> DRPAVVHSVRALMLAERQGGGGSGGGGSGGGGSFFYGKIGECHYLNGTERVRFLDRQIYNRQQFAHFDSDVGKFVADTPLGEPQAEYWNSNAELLENLMNEVDRVCRHNYGILESFTVQRSVEPKVRVSALQSGSLPETD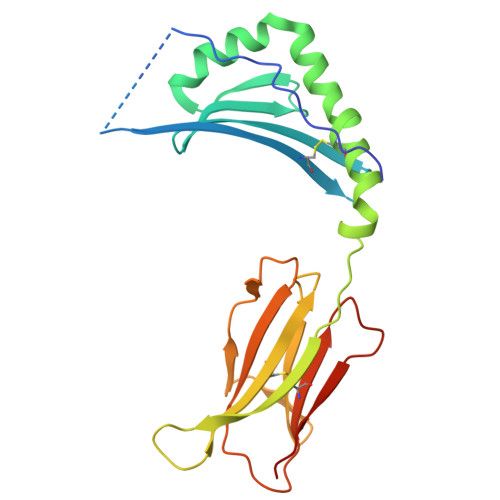RLACYVTGFYPPEIEVKWFLNGREETERVVSTDVMQNGDWTYQVLVVLETVPRRGDSYVCRVEHASLRQPISQAWEPPADAGRSK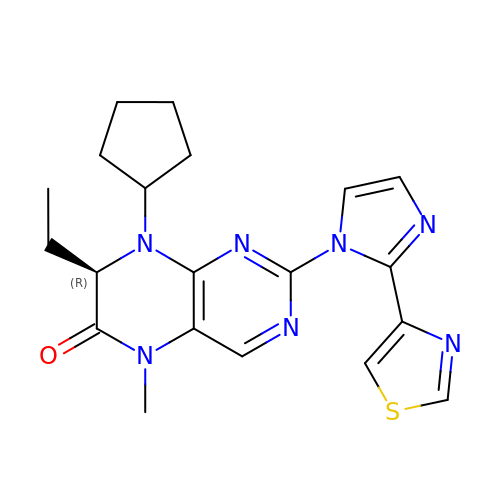(7R)-8-cyclopentyl-7-ethyl-5-methyl-2-[2-(1,3-thiazol-4-yl)-1H-imidazol-1-yl]-7,8-dihydropteridin-6(5H)-one | C20 H23 N7 O S | HGHXLCCYGNWFLX-OAHLLOKOSA-N(3S)-1-[2-(5-chloro-2,4-dimethoxyphenyl)imidazo[1,2-a]pyridin-7-yl]-N-[(pyridin-4-yl)methyl]pyrrolidin-3-amine | C25 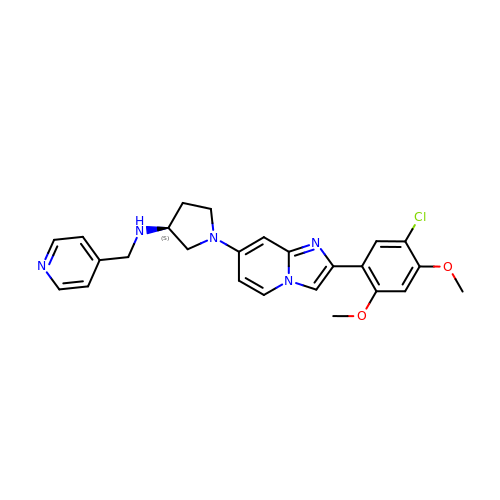H26 Cl N5 O2 | YDTCRGKEOJGNHD-SFHVURJKSA-N> GGACAUAUAAUCGCGUGGAUAUGGCACGCAAGCUUC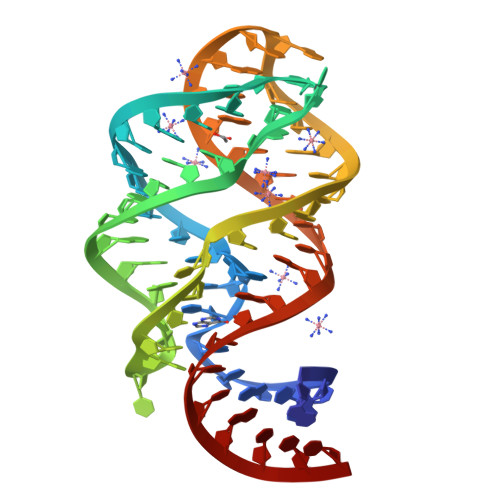UACCGGGCACCGUAAAUGUCCGACUAUGUCC>[2x]AGIKVFGHPASIATRRVLIALHEKNLDF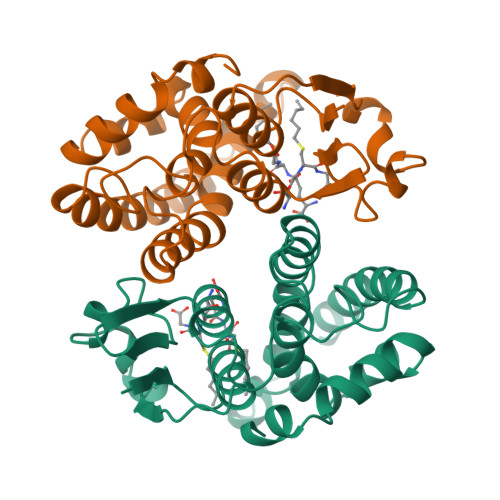ELVHVELKDGEHKKEPFLSRNPFGQVPAFEDGDLKLFESRAITQYIAHRYENQGTNLLQTDSKNISQYAIMAIGMQVEDHQFDPVASKLAFEQIFKSIYGLTTDEAVVAEEEAKLAKVLDVYEARLKEFKYLAGETFTLTDLHHIPAIQYLLGTPTKKLFTERPRVNEWVAEITKRPASEKVQ>[6x]GSSPNLRYPIADVSGGIGMSPNYRFRQSMWIGIVSYSGSGL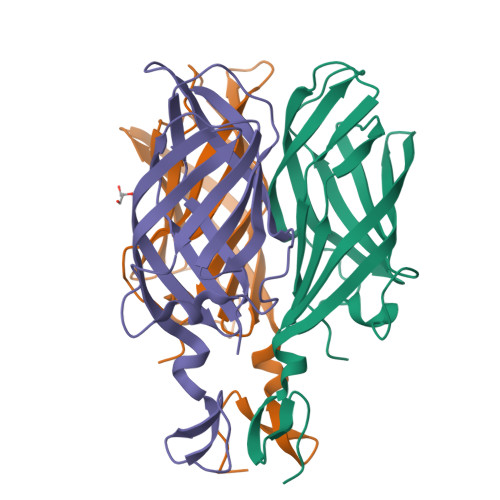NWRVQVNSDIFIVDDYIHICLPAFDGFSIADGGDLSLNFVTGLLPPLLTGDTEPAFHNDVVTYGAQTVAIGLSSGGTPQYMSKNLWVEQWQDGVLRLRVEGGGSITHSNSKWPAMTVSYPRSFT>[2x]MSPRSRLLASSLRGGLLLRPCSARRSTLLNPSPSPLRKAIFHTTSLRAFKNLAEIATSSKEDASSLKPKGKPSPPGDPLATIEKTAAEQRRADWAIIKQMSRYLWPKDSWSDKARVLLALSLLVGGKVLNVHVPFYFREIIDRLNIDVAAVGGTVSAVAGAVIFAYGASRIGAVVSQELRNAVFSSVAQKAIRRVATQTFGHLLNLDLSFHLSKQTGGLTRAIDRGTKGISYLLTSMVFHIVPTALEIGMVCGILTYQFGWEFAAITAATMAAYTAFTITTTAWRTKFRRQANAADNAASTVAVDSLINYEAVKYFNNE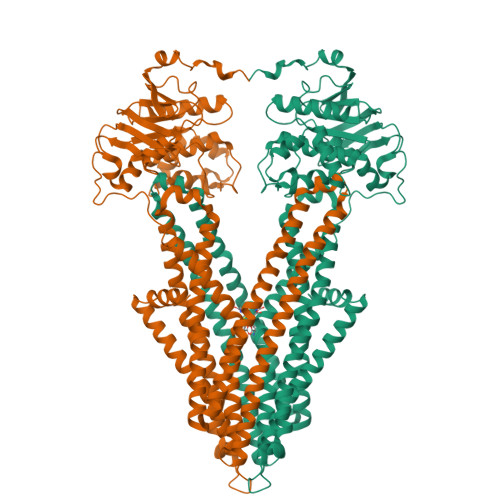AYEIARYDKALQAYERSSIKVATSLAFLNSGQNIIFSSALTLMMWLGARGVLAGDLSVGDLVLINQLVFQLSVPLNFLGSVYRELRQSLLDMETLFDLQKVNVTIREAPNAKPLALPKGGEIRFENVTFGYYPDRPILRNLSLTIPAGKKVAVVGPSGCGKSTLLRLLFRSYDPQQGKIFIDDQDIKSVTLESLRKSIGVVPQDTPLFNDTVELNIRYGNVNATQEQVIAAAQKAHIHEKIISWPHGYQTRVGERGLMISGGEKQRLAVSRLILKDPPLLFFDQATSALDTHTEQALMANINEVVKEKKRTALFVAHRLRTIYDADLIIVLKEGVVVEQGSHRELMERDGVYAELWMAQEMLHQGEAAEEPAEGEKAEEKK>MTPPAPVFSFLFDEKCGYNNEHLLLNLKRDRVESRAGFNLLLAAERIQVGYYTSLDYIIGDTGITKGKHFWAFRVEPYSYLVKVGVASSDKLQEWLRSPRDAVSPRYEQDSGHDSGSEDACFDSSQPFTLVTIGMQKFFIPKSPTSSNEPENRVLPMPTSIGIFLDCDKGKVNFYDMDQMKCLYERQVDCSHTLYPAFALMGSGGIQLEEPITAKYLEYQEDMAENLYFQ[4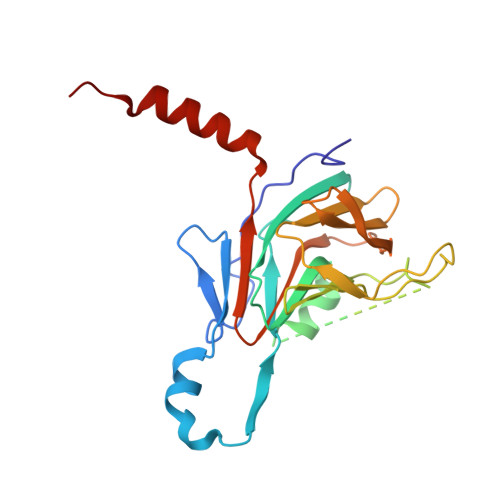x]>MSSILRLDRLRQFIGELATLLDSRPDESTLLAQAHPLLAELVHQDDWLPEDCARPDPQRYQQYLLHVDSRQRFSVVSFVWGPGQITPVHDHRVWGLIGMLRGAEYSQPYAFDAGGRPHPSGARRRLEPGEVEALSPRIGDVHQVSNAFSDRTSISIHVYGANIGAVRRAVFSAEGEEKPFISGYSNSRLPNIWD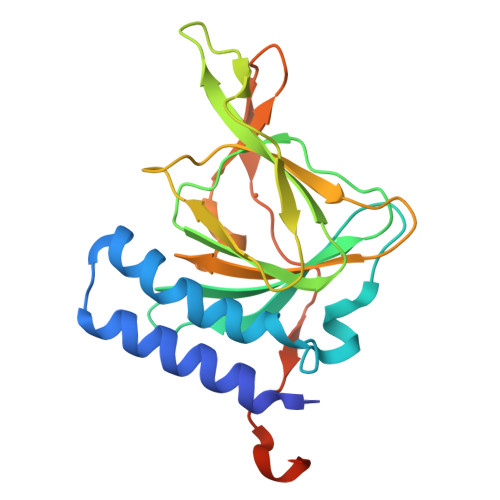LSKENPASAWSHPQFEK[4x]> MSYQTKRNVRREARTLMGRFKAGKLAPVMAVPVKGSEGGMLSQSVSFELDPIAGRMATPITAEMCAVFVPVQACDALKNPEADYAGMTEIVREKLLSGNPLFVLEPETDVSKRCGVNPRRNNGLMRVNEIVRLAHNCAVNFLRRRRYVDAVQLTAANHSTTPAILSQTVLDRFNGALDPDPNVNG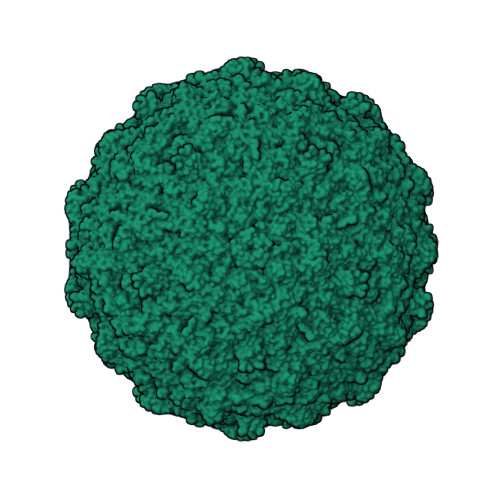AVQLSMPDMRLPVASDAEKAVTAPLTVKRGNENRRLDAGISRLAAAEVAAATDAALYAVFGGREAGNVSLTDFYNAQKMDELTRVMRKICDDNPEYGEEMVLRWAHGLSVDPGRVPFLLAEKSVVLGRQIIGATDTAGVEDGVKRSDMAAQLSFTVPIPTTELGGIIVTFACIKPDETLSSQPHPILADHWRLDNFVADELALDPQPVMARELDYKVAQANETTVVFYTGLNELKKTYVSYGLCRALDPNTVESKNAVWQLEVPLSVTPETVLYPADLPQYPFADQQAEVCTYVVQSTAVMPTPMIFGPSPVEQLAVIETEDLFED> MPPFRQVGEKQLPHEIIFLAWSPKRDLIALVNKAGEVLLHRLANIQRVWSLPPNENTGKEVTCLAWRPDGKILAFGLADTKKVILCDVEKPESLHSFSLETPISCMQWMEVNVENSVLTSFYNAEDEANVLLPKLPALPKNYTATAKIFSEEKSDEILKLLGDARLNALVLGGDSGQIEIYAYGMYKIATISEVYGSCLRLCLSSDLKSLSVVTELTTNNTPEITYFQLDTSLLSDYLPEVTRMARKFTHISTLLQYLQLSLTCMCEAWEEILMQMDSRLTKFVQEKNTTTSVQDEFMQLLLWGKASPELQTLLMNQLTVKGLKKLGQSVESSYSTIQKLVISHLQSGAEALLYHLSELKGMALWRQKYEPLGLDAKAIEDAITAVGSFILKAHELLQVIDSGMKNFKAFFRWLYVAMLRMSEDHVLPELNKMTQKDITFVADFLTEHFNEAPDMYNQKGKYFNVERVGQYLKDEDDILMSPPNIEGNQWFSFLQSSTHLKESPLLFPYYPEKSLHFVKRQMEAIIDRCLTKPAQIIGASVQQKRCLPLYQVSASEEACPRLISLPYLWNDKSQNLHCVMFRMLESSSSKVFILRQPTDLSRSINEALLAVTIGNSLNSSAAEDTETSSYSCLDARFYDEDIITVVLRDNSEPEGKDRVLSQLSLSQLYSDEETEDEFTWDTSKRLEEQHSDIPTRTVFLENQGRLLENMKAHYVSVNGIRKVACVLSSNLRHVRVFEMDA

The anaphase-promoting complex/cyclosome (APC/C) is a large multimeric cullin-RING E3 ubiquitin ligase that functions to regulate cell cycle transitions by ubiquitinating specific cell cycle regulatory proteins and targeting them for proteolysis by the ubiquitin-proteasome system. Only four subunits are directly involved in catalyzing protein ubiquitination (the cullin subunit Apc2 and the RING subunit Apc11) and degron recognition [coactivator subunits (either Cdc20 or Cdh1) and Apc10]. The remaining 85% of the APC/C mass corresponds to scaffolding subunits, of which seven are large multiple repeat motif proteins (Apc1 and Apc3–Apc8). Seeking to obtain insights into these structures at atomic resolution and to assist in the interpretation of cryo-EM reconstructions of the APC/C complex, we determined the crystal structures of full-length Apc4 and the N-terminal domain of Apc5 (Apc5N).

We first determined the crystal structure of Xenopus laevis Apc4 (residues 1–741 that lacked the C-terminal 48 residues that were predicted to be disordered). The protein was overexpressed in the insect cell/baculovirus system and the structure was determined using phases to 3.2 Å resolution derived from multiwavelength anomalous diffraction. Tracing of the polypeptide chain was guided by selenomethionine anomalous signals. Apc4 adopts a bi-domain architecture, dominated by a 360-residue seven-bladed WD40 β-propeller domain (Apc4WD40) split by the HBD (Apc4HBD) predominantly composed of four long α-helices. Apc4HBD is inserted between strands C and D of blade 4 of the WD40 domain, extending away from the wider lower surface of the β-propeller such that, together, the HBD and WD40 domain generate an L-shaped molecule. A second smaller insert between β-strands A and B within blade 3 of Apc4WD40 contacts Apc4HBD. Finally, an insert between β-strands C and D of blade 6 forms an edge β-strand (βE5) with β-strand D of blade 5. Apart from these three insertions, Apc4WD40 resembles a canonical β-propeller architecture as judged by its similarity with other WD40 domain proteins (high DALI Z scores). To our knowledge, the insertion of a helical bundle domain within a WD40 β-propeller domain is novel. Human and X. laevis Apc4 are also very similar, differing only for residues 120–130 (X. laevis Apc4 numbering) within the shorter WD40 insert that is an α-helix in the X. laevis Apc4 structure in contrast to a predominantly disordered loop structure in human Apc4.> MGYYDIDDVLADGTEFPCKFQYDIPGLGYLENNPGRPITKNTKLSLPLWLARILAIVGGDEALVDEEPVPFVE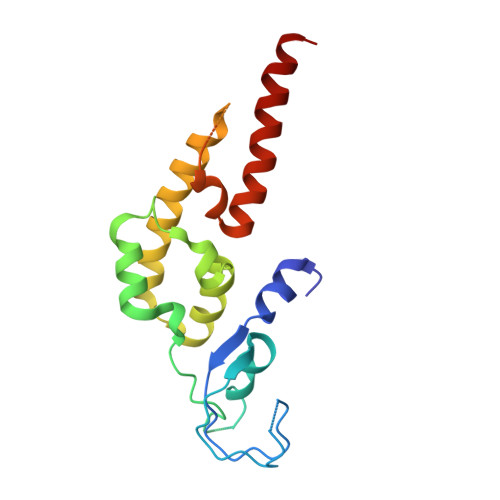LLPPDMFSTKVMNAIKTDPVALDLHSINSHFFSLAIKWIMLFSEKELANVVSELLLQRAQELNHHASSLSIDLNADSTGKNSANTNIATSTFLLKLEEMEKEIYKKSHESYKDTKRWMFKK>MDLFMRIFTIGTVTLKQGEIKDATPS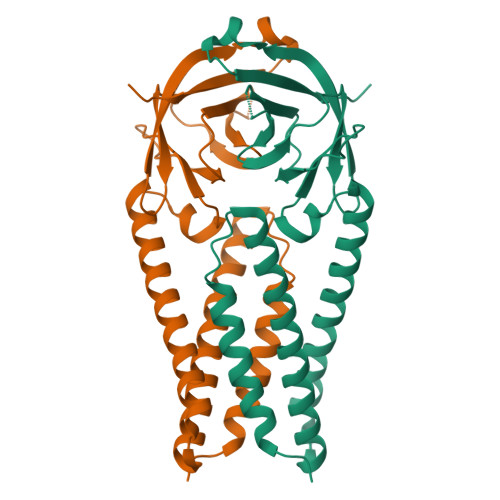DFVRATATIPIQASLPFGWLIVGVALLAVFQSASKIITLKKRWQLALSKGVHFVCNLLLLFVTVYSHLLLVAAGLEAPFLYLYALVYFLQSINFVRIIMRLWLCWKCRSKNPLLYDANYFLCWHTNCYDYCIPYNSVTSSIVITSGDGTTSPISEHDYQIGGYTEKWESGVKDCVVLHSYFTSDYYQLYSTQLSTDTGVEHVTFFIYNKIVDEPEEHVQIHTIDGSSGVVNPVMEPIYDEPTTTTSVPLSNSLEVLFQ[2x]> MNFLRGVMGGQSAGPQHTEAETIQKLCDRVASSTLLDDRRNAVRALKSLSKKYRLEVGIQAMEHLI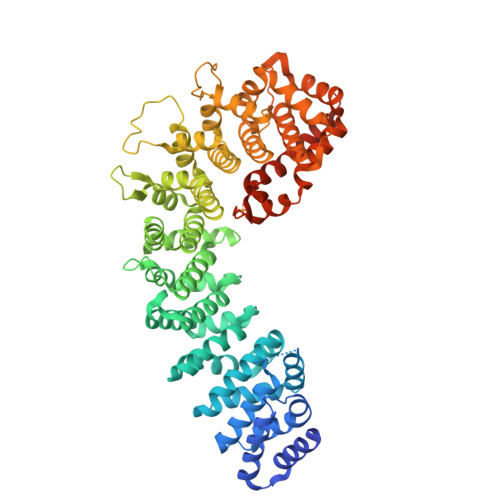HVLQTDRSDSEIIGYALDTLYNIISNDEEEEVEENSTRQSEDLGSQFTEIFIKQQENVTLLLSLLEEFDFHVRWPGVKLLTSLLKQLGPQVQQIILVSPMGVSRLMDLLADSREVIRNDGVLLLQALTRSNGAIQKIVAFENAFERLLDIITEEGNSDGGIVVEDCLILLQNLLKNNNSNQNFFKEGSYIQRMKPWFEVGDENSGWSAQKVTNLHLMLQLVRVLVSPNNPPGATSSCQKAMFQCGLLQQLCTILMATGVPADILTETINTVSEVIRGCQVNQDYFASVNAPSNPPRPAIVVLLMSMVNERQPFVLRCAVLYCFQCFLYKNQKGQGEIVSTLLPSTIDATGNTVSAGQLLCGGLFSTDSLSNWCAAVALAHALQENATQKEQLLRVQLATSIGNPPVSLLQQCTNILSQGSKIQTRVGLLMLLCTWLSNCPIAVTHFLHNSANVPFLTGQIAENLGEEEQLVQGLCALLLGISIYFNDNSLETYMKEKLKQLIEKRIGKENFIEKLGFISKHELYSRASQKPQPNFPSPEYMIFDHEFTKLVKELEGVITKAIYKSSEEDKKEEEVKKTLEQHDSI> MILDTDYITEDGKPVIRIFKKENGEFKIEYDRTFEPYFYALLKDDSAIEEVKKITAERHGTVVTVKRVEKVQKKFLGRPVEVWKLYFTHPQDVPAIRDKIREHPAVIDIYEYDIPFAKRYLIDKGLVPMEGDEELKMLAFAIATLYHEGEEFAEGPILMISYADEEGARVITWKNVDLPYVDVVSTEREMIKRFLRVVKEKDPDVLITYNGDNFDFAYLKKRCEKLGINFALGRDGSEPKIQRMGDRFAVEVKGRIHFDLYPVIRRTINLPTYTLEAVYEAVFGQPKEKVYAEEITTAWETGENLERVARYSMEDAKVTYELGKEFLPMEAQLSRLIGQSLWDVSRSSTGNLVEWFLLRKAYERNELAPNKPDEKELARRRQSYEGGYVKEPERGLWENIVYLDFRSLYPSIIITHNVSPDTLNREGCKEYDVAPQVGHRFCKDFPGFIPSLLGDLLEERQKIKKKMKATIDPIERKLL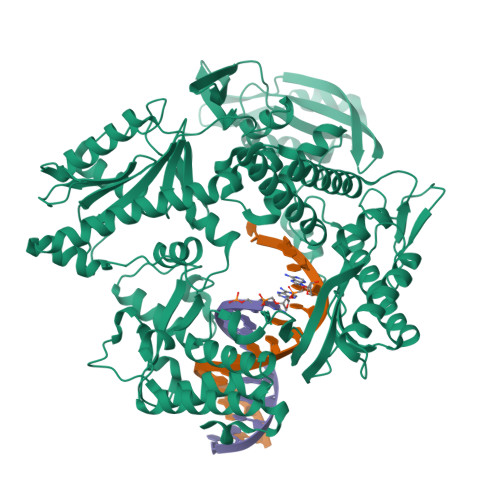DYRQRRIKILANSYYGYYGYARARWYCKECAESVTAWGREYITMTIKEIEEKYGFKVIYSDTDGFFATIPGADAETVKKKAMEFLKYINAKLPGALELEYEGFYKRGFFVTKKKYAVIDEEGKITTRGLEIVRRDWSEIAKETQARVLEALLKDGDVEKAVRIVKEVTEKLSKYEVPPEKLVIHIQITRDLKDYKATGPHVAVAKRLAARGVKIRPGTVISYIVLKGSGRIGDRAIPFDEFDPTKHKYDAEYYIENQVLPAVERILRAFGYRKEDLRYQKTRQVGLSAWLKPKGT>[2x]GU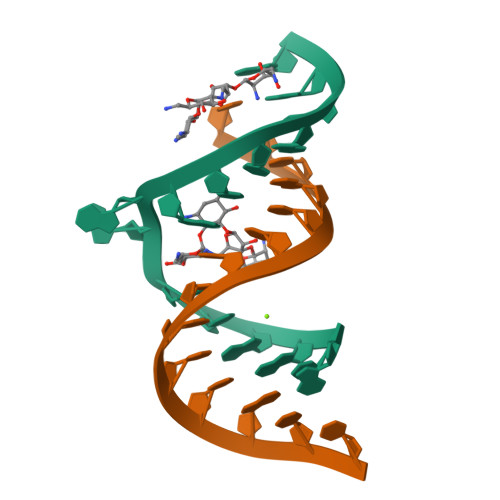GGUGAAGUCGCGG;>[2x]CGCGUCACACCACC>GSALTVRDWPALEALAKTMPADAGARAMTDDDLRAAGVDRRVPEQKLGAAIDEFASLRLPDRIDGRFVDGRRANLTVFDDARVAVRGHARAQRNLLERLETELLGGTLDTAGDEGGIQPDPILQGLVDVIGQGKSDIDAYATIVEGLTKYFQSVADVMSKLQDYISAKDDK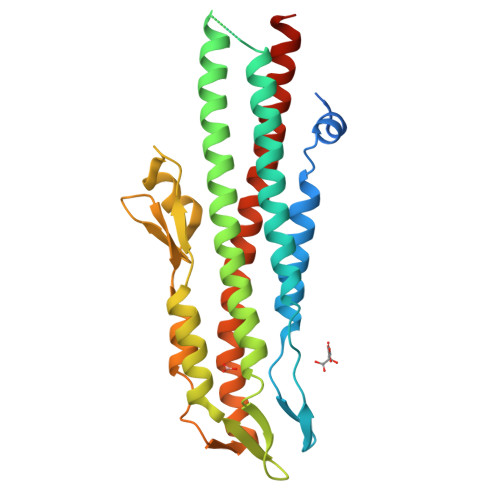NMKIDGGKIKALIQQVIDHLPTMQLPKGADIARWRKELGDAVSISDSGVVTINPDKLIKMRDSLPPDGTVWDTARYQAWNTAFSGQKDNIQNDVQTLVEKYSHQNSNFDNLVKVLSGAISTLTDTAKSYLQI[2x]>MVDAAQYFPGTWEFRFRSSDGKEYRGTVEMQPRTPTEIEIRFKGQSSDGRPVEGRGSIEVRSPYEYRFEMQSSDGARWEGTLQVRSPDSVE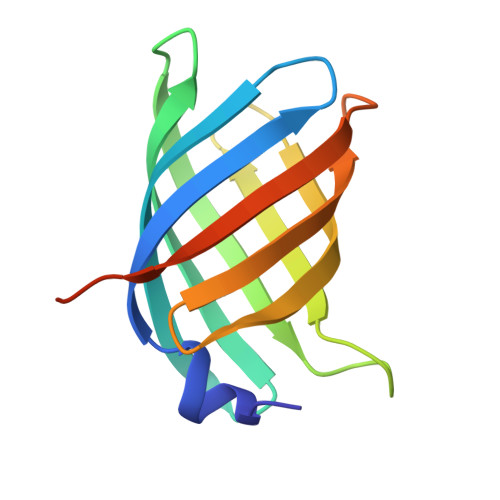VRFKSSDGREYSGEFRRQEGSLEHHHHHH[2x]>[4x]MIGRLRGIIIEKQPPLVLIEVGGVGYEVHMPMTCFYELPEAGQEAIVFTHFVVREDAQLLYGFNNKQERTLFKELIKTNGVGPK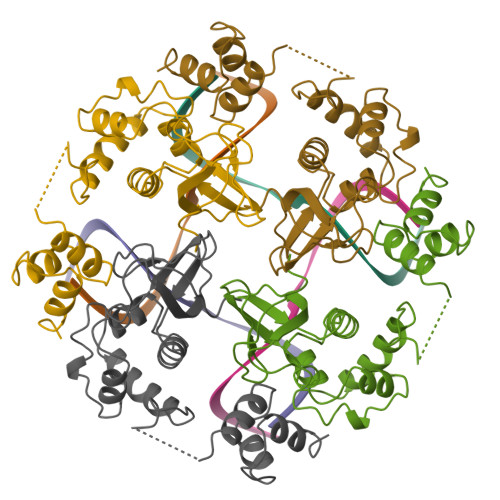LALAILSGMSAQQFVNAVEREEVGALVKLPGIGKKTAERLIVEMKDRFKGLHGDLFTPAADLVLTSPASPATDDAEQEAVAALVALGYKPQEASRMVSKIARPDASSETLIREALRAAL> EWTGDYENIGYFSHEVISEFHVGQIDGG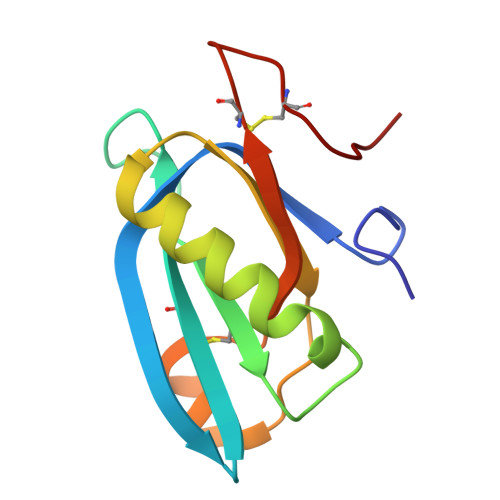AYFCIKAVKADGSRSTPLIACSVSNESVWAPSFKVLLEQARYFYVTEQSVRIYYDHNVWTNQPFVNTFSTNALVGLSSCSAATDCFGPGKP>[6x]GTGAMKD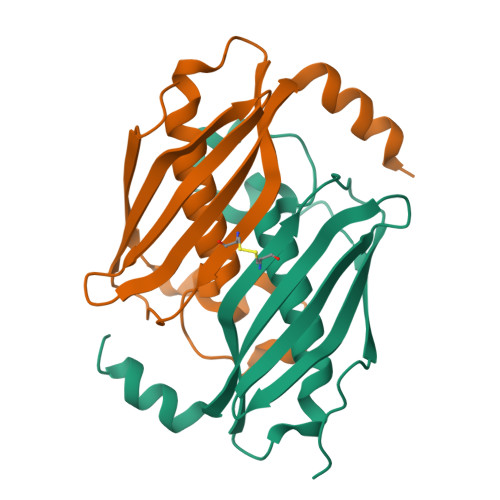GMRVGERFTHDFVVPPHKTVRHLYPESPEFAEAPEVFATGFMVGLMEWACVRAMAPYLEPGEGSLGTAICVTHTAATPPGLTVTVTAELRSVEGRRLSWRVSAHDGVDEIGSGTHERAVIHLEKFNAKVRQKTPAG> GSHMASSESTEEKPDTDLADKYASGNSEISGQELRGLRDAIGDDASPEDILALVQEKIKDPALQSTALDYLVQTTPPSQGKLKEALIQARNTHTEQFGRTAIGAKNILFASQEYADQLNVSPSGLRSLYLEVTGDTHTCDQLLSMLQDRYTYQDMAIVSSFLMKGMATGLKRQGPYVPSAQLQVLMTETRNLQAVLTSYDYFESRVPILLDSLKAEGIQTPSDLNFVKVAESYHKIINDKFPTASKVEREVRNLI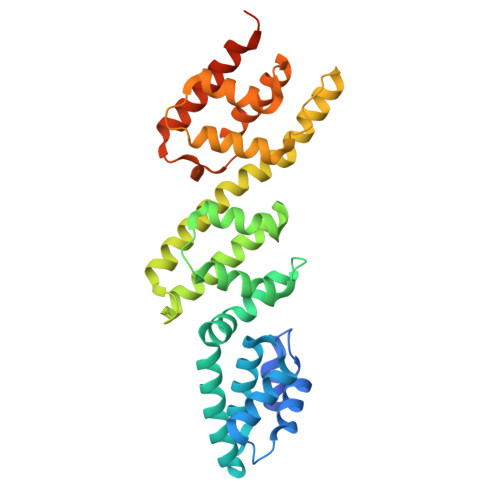GDDVDSVTGVLNLFFSALRQTSSRLFSSADKRQQLGAMIANALDAVNINNEDYPKASDFPKPYPWS>[4x]ATQGVFTLPANTQFGVTAFANSAGTQTVNVQVNNETVATFTGQSTNNAIIGSKVLNSGGGGKVQILVSVNGRSSDLVSAQVILANELNFALVGSEDSTDNDYNDAVVVINWPLG

Two extracellular carbohydrate-binding proteins, LecA (PA-IL) and LecB (PA-IIL), are virulence factors and necessary for adhesion and biofilm formation. LecA binds to d-galactose; LecB from the strain PAO1 shows high binding affinities for l-fucose and reduced binding to d-mannose and their glycoconjugates. The genes of both P. aeruginosa lectins lecA and lecB are part of the core genome25 and while LecA is highly conserved, LecB shows sequence variation in 15 amino acids in PA14 compared to PAO1. Despite high sequence variations, biophysical characterization uncovered that both variants possess very similar glycan binding preferences, although very surprisingly LecBPA14 generally displays 2- to 7-fold higher affinities.

Additionally, a direct contact of these hydroxy groups with D96, D99 and the C-terminal G114 of the neighboring monomer is observed. In the fucose-containing ligands the C-6 methyl group is embedded in a lipophilic pocket formed by T45 and A23. This latter variation in the CRD, S23A, allows additional van der Waals interactions between A23 and aglycones of the Ca2+-coordinated carbohydrate moiety. In contrast to LecBPAO1, the G97S variation in LecBPA14 offers an additional hydroxy group with hydrogen bonding potential in the CRD. In each of the three LecBPA14 complexes, the carbohydrate ligands establish one water-mediated hydrogen bond with S97. In contrast to LecBPAO1, the binding of methyl α-l-fucoside (2, Kd 202 nM for LecBPA14), methyl α-d-mannoside (5, Kd 16 μM for LecBPA14) and the H-type II antigen (15, Kd 199 nM for LecBPA14) revealed reduced enthalpic contributions to binding compensated with favorable entropic contribution for LecBPA14. Therefore, both variations are likely to contribute to the increased affinity of LecBPA14 for its ligands compared to LecBPAO1.> GDRVADVIESSIGDSVSRALTRALPAPTGQDTQVSSHRLDTGKVPALQAAEIGASSNASDESMIETRCVLNSHSTAETTLDSFFSRAGLVGEIDLPLEGTTNPNGYANWDIDITGYAQMRRKVELFTYMRFDAEFTFVACTPTGQVVPQLLQYMFVPPGAPEPDSRESLAWQTATNPSVFVKLSDPPAQVSVPFMSPASAYQWFYDGYPTFGEHKQEKDLEYGACPNNMMGTFSVRTVGTSKSKYPLVIRIYMRMKHVRAWIPRPMRNQNYLFKANPNYAGNFIKPTGASRTAITTL;> SPSAEACGYSDRVAQLTIGNSTITTQEAANIIVGYGEWPSYCSDSDATAVDKPTRPDVSVNRFYTLDTKLWEKSSKGWYWKFPDVLTETGVFGQNAQFHYLYRSGFCIHVQCNASKFHQGALLVAVLPEYVIGSVAGGTGTEDTHPPYKQTQPGADGFELQHPYVLDAGIPISQLTVCPHQWINLRTNNCATIIVPYINALPFDSALNHCNFGLLVVPISPLDYDQGATPVIPITITLAPMCSEFAGLRQAVTQ;> GFPTELKPGTNQFL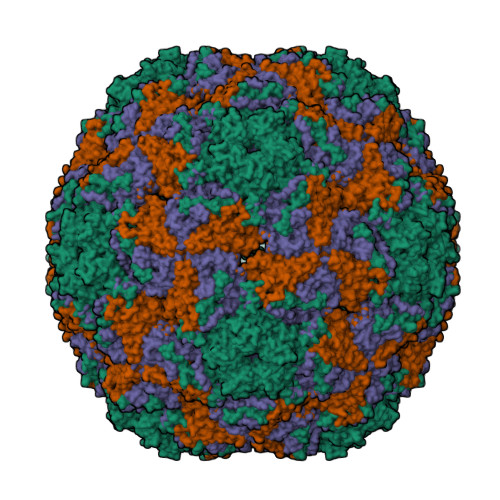TTDDGVSAPILPNFHPTPCIHIPGEVRNLLELCQVETILEVNNVPTNATSLMERLRFPVSAQAGKGELCAVFRADPGRSGPWQSTLLGQLCGYYTQWSGSLEVTFMFTGSFMATGKMLIAYTPPGGPLPKDRATAMLGTHVIWDFGLQSSVTLVIPWISNTHYRAHARDGVFDYYTTGLVSIWYQTNYVVPIGAPNTAYIIALAAAQKNFTMKLCKDASDILQTGTIQ;> MGSQVSTQRSGSHENSNSATEGSTINYTTINYYKDSYAATAGKQSLKQDPDKFANPVKDIFTEMAAPLK> GPSIEYTATALQERCGSFCSASDILGFRAIEHLRRAK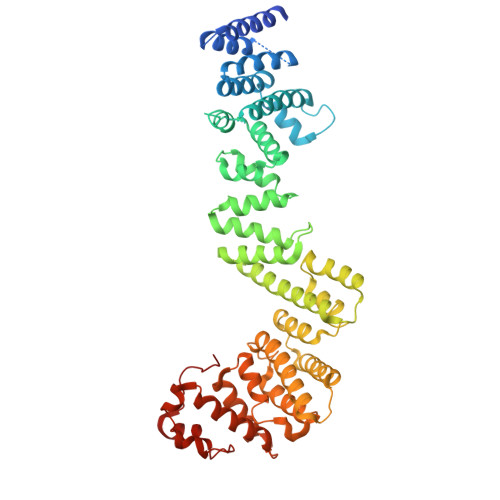EIGLRNYDSLNYHLKNATALLEQIVDDLSIEKLKEAVSMMLSVNYYPKSIEFLLNIANSMDKGKLACQYVANGFLENDDRKQYYDKRILVYDLVFDTLIKVDELAEKKQSSKTQNQISISNDDEVKLRQKSYEAALKYNDRLFHYHMYDWLVSQNREEKLLDIETPFILPYLMEKAGSSLKISNILWVYYSRRSKFFESAEILYRLATSNFDITLFERIEFLSRANGFCNSVSPLSQKQRIVQLASRIQDACEVAGIQGDILSLVYTDARIDSAIKDELIKTLDGKILSTSELFNDFAVPLSYHEIALFIFKIADFRDHEVIMAKWDELFQSLRMEFNNTGKKEDSMNFINLLSNVLIKIGKNVQDSEFIFPIFELFPIVCNFFYETLPKEHIVSGSIVSIFITAGVSFNKMYYILKELIETSDSDNSVFNKEMTWLIHEWYKSDRKFRDIISYNDIIHLKEYKIDNDPIEKYVKNSGNNLGICFYKE>[3x]MGSDKIHHHHHHMKTFHLTTQSRDEMVDITS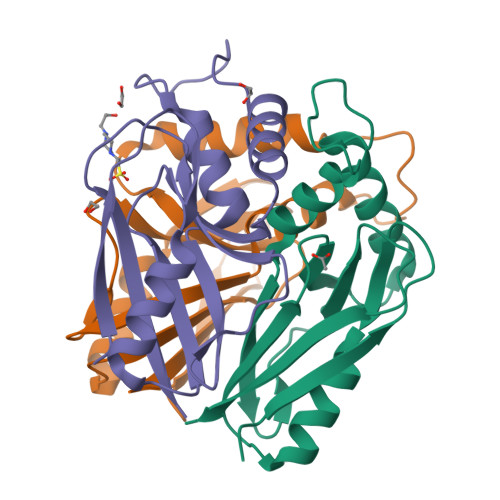QIETWIRETGVTNGVAIVSSLHTTAGITVNENADPDVKRDMIMRLDEVYPWHHENDRHMEGNTAAHLKTSTVGHAQTLIISEGRLVLGTWQGVYFCEFDGPRTNRKFVVKLLTD>MSLTEPRIVATYHIASDAERIEQRALALAIEQSVECPLEAIGDPAIVANIVGRVEDVAELQPGRYAVRIGLAAATAPAEPGQLLNMLFGNSSIQPDIALADVELPAHYLTAFGGPRVGLAGIRTLTGAQSRALTASALKPQGLSP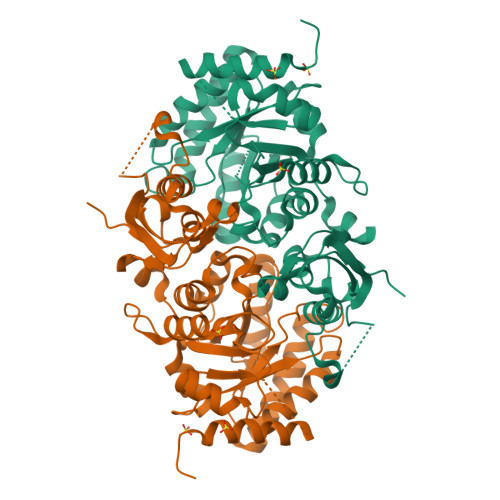AALASIAHQLALGGVDLIKDDHGLADQAFSPFAERAAAVGKAVREANAARGGRTLYAPNISGTLDDMRRQLGVIRDEGIGAVLVAPMIVGVSNFHAIVKEAAGLVVVAHPAMAGAAKIAAPLLLGRLFRLFGADATVFPNYGGRFAYSTASCLALAQAARDPFGKLNACIPTPAGGIMLQRVNELLRFYGQDVMLLIGGSLLASRERLTEQASRFVNKVADYGQREGHHHHHH[2x]> SYDPDNKEE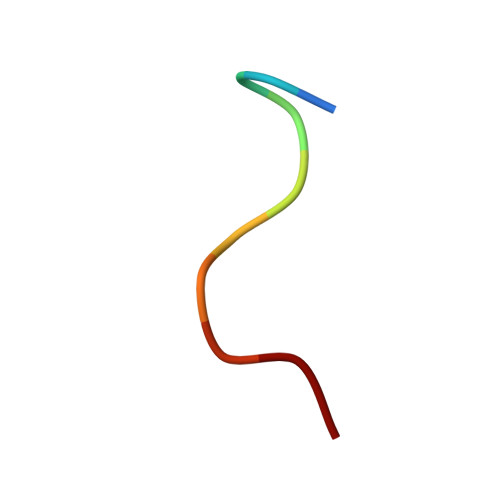R>[4x]WTGEDSAEPNSDSAEWIRDMYAKVTEIWQEVMQRRDDDGTLHAACQVQPSATLDAAQ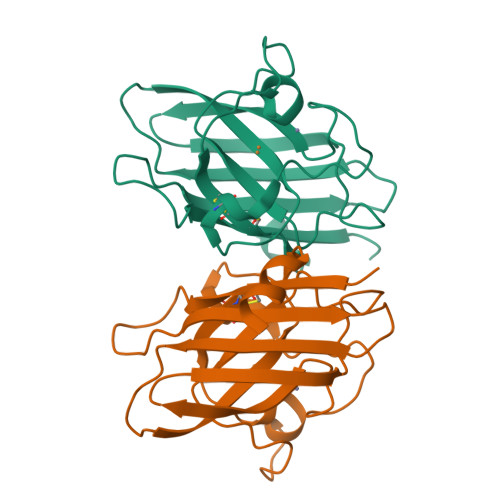PRVTGVVLFRQLAPRAKLDAFFALEGFPTEPNSSSRAIHVHQFGDLSQGCESTGPHYNPLAVPHPQHPGDFGNFAVRDGSLWRYRAGLAASLAGPHSIVGRAVVVHAGEDDLGRGGNQASVENGNAGRRLACCVVGVCGPGLWERQAREHSERKKRRRESECKAA> AFSRPGLPVEYLQVPSASMGRDIKVQFQGGGPHAVYLLDGLRAQDDYNGWDINTPAFEEYYQSGLSVIMPVGGQSSFYTDWYQPSQSNGQNY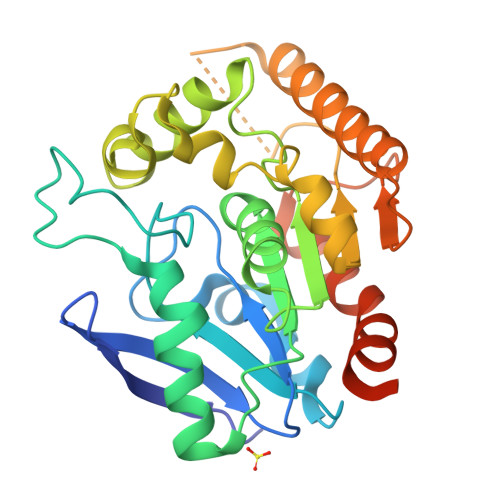TYKWETFLTREMPAWLQANKGVSPTGNAAVGLSMSGGSALILAAYYPQQFPYAASLSGFLNPSEGWWPTLIGLAMNDSGGYNANSMWGPSSDPAWKRNDPMVQIPRLVANNTRIWVYGGNGTPSDLGGDNIPAKFLEGLTLRTNQTFRDTYAADGGRNGVFNFPPNGTHSWPYWNEQLVAMKADIQHVLNGATPPAAPAAPAAHHHHHH The cadherin-catenin cell adhesion complex is the major building block of AJs, and has a crucial function in the dynamic behaviors of epithelial cells, such as cell polarization and cell rearrangements. The structure of α-catenin (100 kDa) consists of three distinct domains. The C-terminal actin-binding domain (ABD) (28 kDa), which is connected to the rest by a flexible P-linker region28 (2 kDa), directly binds to F-actin, and closely resembles the vinculin ABD (vin-ABD). The direct interaction between α-catenin and F-actin was demonstrated to be a catch bond, an interaction that is stabilized by increased force.

To assess whether the α1-helix affects the α-catenin-F-actin interaction, we performed in vitro actin cosedimentation assays with three ABD variants of αE- and αN-catenin (αE-catenin residue numbers are shown): a wild type form of ABD (ABD-WT; residues 652-906), an ABD with a structure-guided helix-1 mutation (H1) designed to unfold α1-helix (ABD-H1; RAIM670-673GSGS), and an ABD with a partially deleted α1-helix (ABD-Δα1; residues 671-906). We observed a nearly two-fold increase in the cosedimented amount of either ABD-H1 or ABD-Δα1 compared to ABD-WT. To examine the structural details of αcat-ABD with enhanced F-actin binding, we determined crystal structures of αNcat-ABD-H1. However, unlike the monomeric αNcat-ABD-WT structure, αNcat-ABD-H1 crystallized as a homodimer connected by two βH motifs. The dimer interface involves L807N of the βH, which mimics M673N of α1-helix interacting with the hydrophobic patch in the αNcat-ABD-WT structure. Moreover, the observation of αNcat-ABD-H1 dimerization, which occludes 3100 Å2 of solvent-accessible surface, in two distinct crystal forms provides a basis for further examining the physiological relevance of this ABD-dimer interface. Our NMR analysis of αNcat-ABD-H1 in solution showed that concentration-dependent chemical shift perturbations (CSPs) mostly occurred in the βH motif. In addition, we performed chemical shift (CS)-based Rosetta comparative modeling (CM)48 to show that V796N of αNcat-ABD-WT remained in the cryptic state, whereas αNcat-ABD-H1 displayed a large conformational change that exposed V796N on the surface, resembling V796 in the crystal structure of αEcat-ABD-WT. Our αNcat-ABD-H1 crystal structures revealed an unexpected ABD homodimerization, which can facilitate F-actin bundling in vitro. It involves the βH motif forming an extensive dimer interface with the hydrophobic patch uncovered by α1-helix unfolding.

>GSSRTSVQTEDDQLIAGQSAGSGSAQLPQEEKAKIAEQVEIFHQEKSKLDAEVAKWDDSGNDIIVLAKQMCMIMMEMTDFTRGKGPLKNTSDVINAAKKIAEAGSRMDKLARAVADQCPDSACKQDLLAYLQRIALYCHQLNICSKVKAEVQNLGGELIVSGLDSATSLIQAAKNLMNAVVLTVKASYVASTKYQKVYGTAAVNSPVVSWKMKAPEKKPLVKREKPEEFQTRVRRGSQKKHISPVQALSEFKAMDSF[2x]>MGHHHHHHSSYTSITKLTNLTEFRNLIKQNDKLVIDFYATWCGPCKMMQPHLTKLIQAYPDVRFVKCDVDESPDIAKECEVTAMPTFVLGKDGQLIGKIIGANPTALEKGIKDL[2x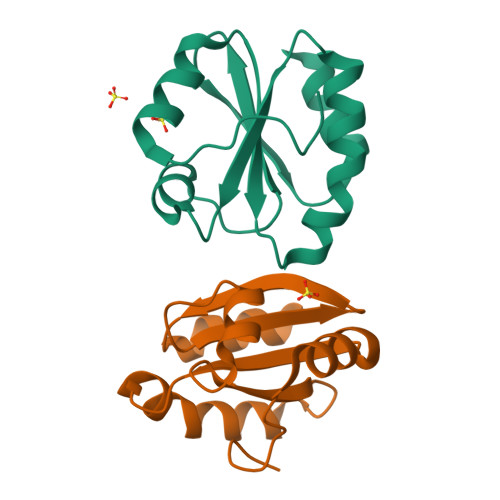]> MRRFLPSSVAAWGAGRVLQCAAEWYHMPGWKTQSSTKDARSREQRERDRKARQIEKLPRPEALHDFQYPYEKTILSDSMFEYPVYETELDTPQLFNLTPPPDFFIYWNATDFDRTAYPPVPEDDHRVLVPSSQSPRWIEHRARLLQYLRKHEIMPHYVPHIHANVNLSVVFPGQYNTRARLTDENGDKIPPPPAQTKMTPRNFWFTAHCGNYMELTDVQQPPS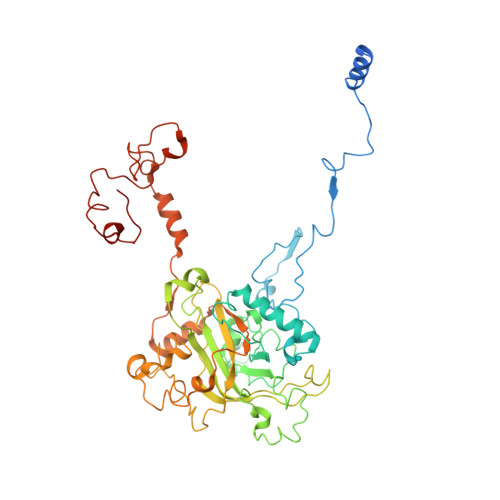VFFFEEAPAAASAASDAGEAGDAANKQSSHAAVNYYTFVMLSPDYPYRVPLLQDRHKADRGFFLNYMVANLRAPQAVSTVDGAVVDTEGLQSKGDVVVPYVAPLPTEDAGTTRHLCLLFKQTGHVPSVKPMTATEEQRDFPLAQRSNYRLHSALTKQTGLKMPPSASTACLASLRSVERAIPADPCAVSFFTTKWDIQVQEYYEKVGLPEPAAPVDEEIEALLEFHAMRPEKLRVRARHRPDGSVNMGDDPNFWAQALPTRAMDGSMQRGLGWSRRTTMGANGVPVVYPH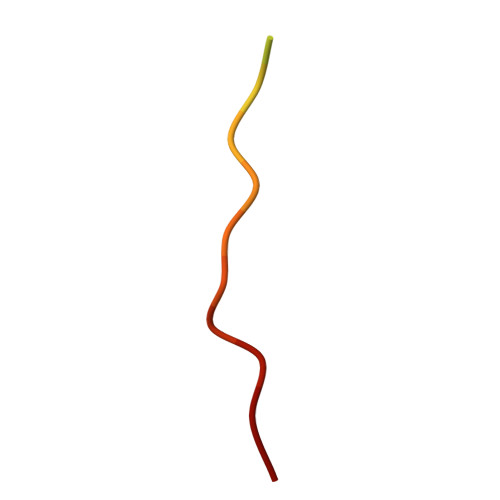> SKPIDHSTITSWVSPDFDTA5'-O-[HYDROXY(PHENYLACETYL)PHOSPHORYL]ADENOSINE | C18 H20 N5 O8 P | 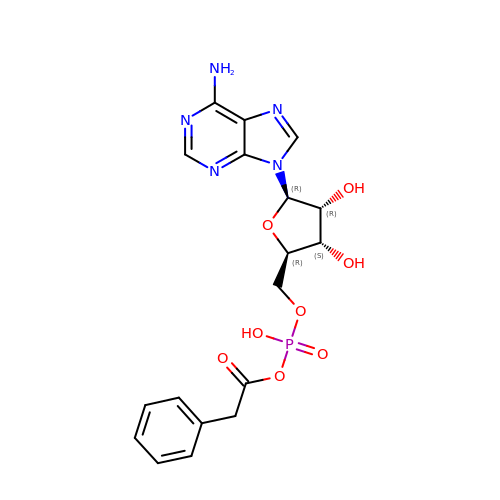VUKDZGAUWUDQRZ-XKLVTHTNSA-N L-alaninamide | C3 H8 N2 O | 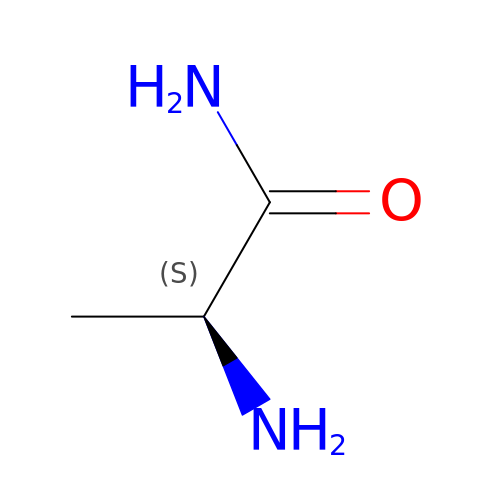HQMLIDZJXVVKCW-REOHCLBHSA-N>[4x]AESLPDLKIEKLDEGVYVHTSFEEVNGWGVVPKHGLVVLVNAEAYLIDTPFTAKDTEKLVTWFVERGYKIKGSISSHFHSDSTGGIEWLNSRSIPTYASELTNELLKKDGK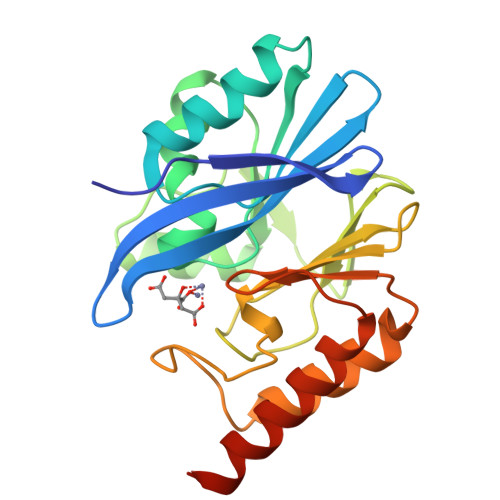VQATNSFSGVNYWLVKNKIEVFYPGPGHTPDNVVVWLPERKILFGGCFIKPYGLGNLGDANIEAWPKSAKLLKSKYGKAKLVVPSHSEVGDASLLKLTLEQAVKGLNESKKPSKPSN> PRERPHTSGHHGAGEARATAPSTVSPYGPEARAELSSRLTTLRNTLAPATNDPRYLQACGGEKLNRFRDIQCRRQTAVRADLNANYIQVG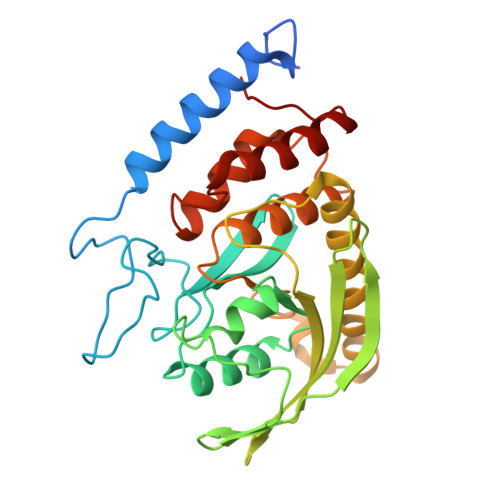NTRTIACQYPLQSQLESHFRMLAENRTPVLAVLASSSEIANQRFGMPDYFRQSGTYGSITVESKMTQQVGLGDGIMADMYTLTIREAGQKTISVPVVHVGNWPDQTAVSSEVTKALASLVDQTAETKRNMYESKGSSAVADDSKLRPVIHSRAGVGRTAQLIGAMCMNDSRNSQLSVEDMVSQMRVQRNGIMVQKDEQLDVLIKLAEGQGRPLLNS Synthesis of phosphatidyl inositol is dependent on free myo-inositol, generated through dephosphorylation of myo-inositol-1-phosphate by inositol monophosphatase (IMPase). In contrast, SuhB appears to be a bona fide IMPase with little or no activity towards fructose-1,6-bisphosphate. Like the human orthologue, SuhB is activated by Mg2+, and inhibited by lithium. Apart from minor discrepancies, the SuhB monomer is identical in fold to eukaryotic IMPases, with RMS deviations between Cα positions of superimposed backbone structures ranging from 1.09 Å to 1.15 Å.

The structure of M. tuberculosis SuhB was determined by molecular replacement to a resolution of 2.6 Å. The asymmetric unit of the crystal lattice contains three independent copies of the SuhB monomer forming two crystallographically distinct dimers: chains A and C associate as one dimer, whereas chain B forms an analogous dimer with one of its symmetry mates. The dimer observed in the crystal structure of SuhB is primarily mediated by helices α6 in layer V and the β-sheet in layer IV, which extends across the interface. Due to the absence of divalent metal ions and of substrate in the active site, the loop connecting helices α1 and α2 is disordered (residues 35–53 missing), as is much of the loop connecting strands β3 and β4 (residues 85–96 missing). The active site of SuhB is situated in a cavity carved out at the N-terminal end of helix α7, sandwiched between layers II and IV. Due to the disordered α1-α2 loop – referred to as the 'mobile loop' – the active site in SuhB appears wide open to solvent. Structural elements of the active site required for metal and substrate binding include the IMPase signature motif 104DPXDGT109 (superscripts denote residue numbers of the SuhB sequence) between strand β4 and helix α4, the 82GEEG85 motif at the 'tip' of the β3-β4 loop, the 209G [ST]AA212 motif in the β10-α7 loop, in addition to Glu228 in β11 and the 234WDXA237 motif in helix α8. All conserved side chains forming the metal binding sites or contacting inositol-1-phosphate are seen in essentially the same conformation as in the human/bovine enzyme, with the exception of Glu83: as a consequence of disorder in a large part of the β3-β4 loop, Glu83 (h_70) in subunit A points outward rather into the active site. The interface of the SuhB dimer buries a total of 2696 Å2 of solvent accessible surface, calculated using the PISA interface server, or 1348 Å2 per monomer. The present data support a model of Mg2+-dependent dimerization, where loading of the three catalytic metal sites in the active site induces ordering of the mobile loop, promoting dimerization likely by expanding the dimer interface.

>[3x]MTRPDNEPARLRSVAENLAAEAAAFVRGRRAEVFGISRAGDGDGAVRAKSSPTDPVTVVDTDTERLLRDRLAQLRPGDPILGEEGGGPADVTATPSDRVTWVLDPIDGTVNFVYGIPAYAVSIGAQVGGITVAGAVADVAARTVYSAATGLGAHLTDERGRHVLRCTGVDELSMALLGTGFGYSVRCREKQAELLAHVVPLVRDVRRIGSAALDLCMVAAGRLDAYYEHGVQVWDCAAGALIAAEAGARVLLSTPRAGGAGLVVVAAAPGIADELLAALQRFNGLEPIPDALEHHHHHH> SHHHHHHHHHSGGGSGGGIEGRVERDKYANFTINFTMENQIHTGMEYDNGRFIGVKFKSVTFKDSVFKSCTFEDVTSVNTYFKNCT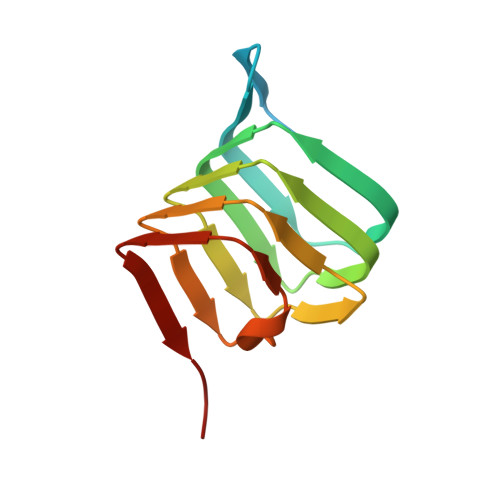FIDTVFDNTDFEPYKFIDSEFKNCSFFHNKT> UCGUAACC;> CCCUCU;> GGUUUGGAGGGAAAAGUUAUCAGGCAUGCACCUGGUAGCUAGUCUUUAAACCAAUAGAUUGCAUCGGUUUAAAAGGCAAGACCGUCAAAUUGCGGGAAAGGGGUCAACAGCCGUUCAGUACCAAGUCUCAGGGGAAACUUUGAGAUGGCCUUGCAAAGGGUAUGGUAAUAAGCUGACGGACAUGGUCCUAACCACGCAGCCAAGUCCUAAGUCAACAGAUCUUCUGUUGAUAUGGAUGCAGUUCACAGACUAAAUGUCGGUCGGGGAAGAUGUAUUCUUCUCAUAAGAUAUAGUCGGACCUCUCCUUAAUGGGAGCUAGCGGAUGAAGUGAUGCAACACUGGAGCCGCUGGGAACUA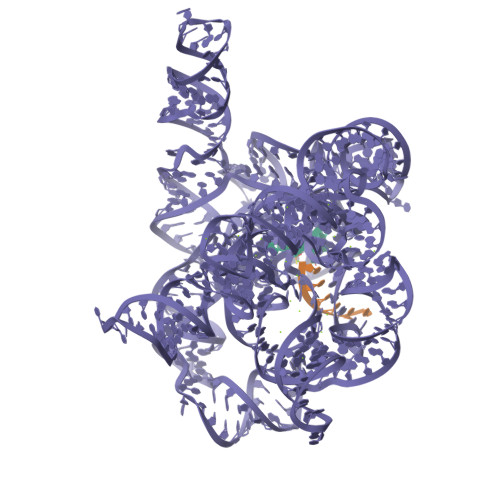AUUUGUAUGCGAAAGUAUAUUGAUUAGUUUUGGAG> AEQKTLHIYNWTEYIAPDTVANFEKETGIKVVYDVFDSNEVLEGKLMAGSTGFDLVVPSAYFLERQLTAGVFQPLDKSKLPEWKNLDPELLKLVAKHDPDNKFAMPYMWATTGIGYNVDKVKAVLGENAPVDSWDLILKPENLEKLKSCGVSFLDDPEEVFATVLNYLGKDPNSTKADDYTGPATDLLLKLRPNIRYFHSSQYINDLANGDICVAIGWAGSVWQASNRAKEAKNGVNVSFSIPKEGAMAWFDVFAMPADAKNKDEAYQFLNYLLRPDVVAHISDHVFYANANKAATPLVSAEVRENPGIYPPADVRAKLFTQKVQDPKIDRVRTRAWTKVKSGKLEHHHHHH

To gain insight into the evolution and designability of ligand binding and specificity, we analyzed the homologous PBPs, PotF and PotD, which are Escherichia coli putrescine (PUT)-binding protein and spermidine (SPD)-binding protein, respectively. They constitute the first elements of two separate multicomponent uptake systems (PotFGHI and PotABCD) to transport the cationic polyamines PUT and SPD across the cellular membrane. Still, the protein-binding modes differ: PotF shows affinity for PUT and SPD, whereas PotD exclusively binds SPD. Prior to this work, we grafted the seven differences in amino acids from PotD binding pocket onto PotF; this resulted in PotF_SPD, which will be referred to as PotF/D throughout this work to keep naming for mutants more concise.

PotF/D solely binds SPD, whereas PUT affinity is abolished. The observation that SPD affinity was solely maintained and PotF/Ds crystal structure adopted a semiclosed state led us to the approaches presented in this work. Closer examination of PotF/D revealed that two mutations interfere with wildtype-like salt bridge formation. Although D39E would increase the length of the one residue involved in the proximal salt bridge and partially open the structure, the exchange from Asp to Glu still allows salt bridge formation in general. However, the second mutation S87Y seemed to have a much bigger impact on the ligand recognition of PotF as shown in the prior analysis. In PotD, this Tyr faces inward into the binding pocket to coordinate N3 of SPD. In contrast, when introduced in PotF/D, this Tyr turns outward and disrupts the salt bridge between E184 and R91. This observation explains the negative influence of S87Y on polyamine binding in general as well as the lack of affinity improvement in PotF/D, as the Tyr does not only disrupt the salt bridge and thereby obstructs complete closure but also is not able to coordinate N3 of SPD. In PotF, this Phe points inside the binding pocket, but in PotF/D, its rotamer is vertically flipped by ∼180°. It appears that F88 and Y87 repel each other in PotF/D, driving both residues away from the binding pocket and eliminating PotD-like positioning of Y87.> QTRHVKNYHSRSESTVENFLCRSACVFYTTYRNHGTDGDNFGYWVISTRQVAQLRRKLEMFTYARFDLELTFVITSTQEQSTIQGQDSPVLTHQIMYVPPGGPVPTKVNSYSWQTSTNPSVFWTEGSAPPRMSIPFISIGNAYSMFYDGWAKFDKQGTYGINTLNNMGTLYMRHVNDGSPGPIVSTVRIYFKPKHVKTWVPRPPRLCQYQKAGNVNFEPTGVTESRTDITTMQ;> RVRSITLGNSTITTQECANVVVGYGVWPTYLNDDEATAEDQPTQPDVATCRFYTLESVMWQQSSPGWWWKFPDALSNMGLFGQNMQYHYLGRAGYTVHVQCNASKFHQGCLLVVCVPEAEMGCATLANKPDQKSLSNGETANMFESQNSTGQTAVQANVINAGMGVGVGNLTIFPHQWINLRTNNSATIVMPYINSVPMDNMFRHNNFTLMIIPFAPLSYSTGATTYVPITVTVAPMCA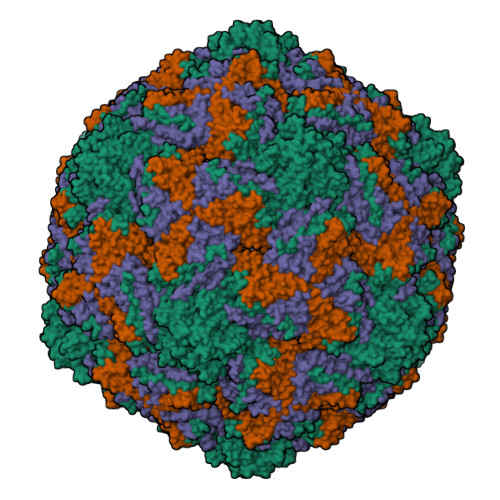EYNGLRLAG;> GLPTMLTPGSNQFLTSDDFQSPSAMPQFDVTPEMDIPGQVNNLMEIAEVDSVVPVNNTEGKVLSIESYQIPVQSNSTNGSQVFGFPLMPGASSVLNRTLLGEILNYYTHWSGSIKLTFMFCGSAMATGKFLLAYSPPGAGAPTTRKEAMLGTHVIWDVGLQSSCVLCIPWISQTHYRYVVVDEYTAGGYITCWYQTNIVVPADTQSDCKILCFVSACNDFSVRMLKDTPFIKQDNFYQ> GSPGISGGGGGILSLLCVGVKKAKFDGAQEKFNTYVTLKVQNVESTTIAVRGSQPS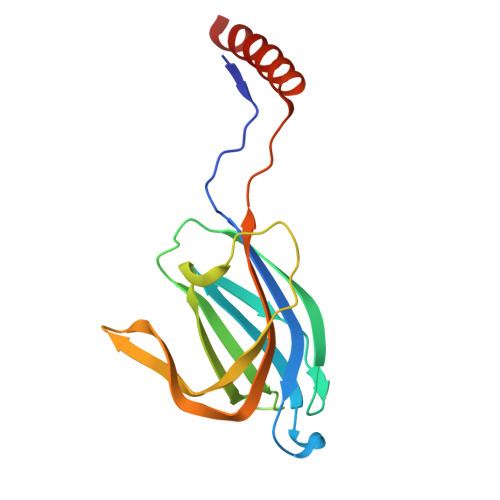WEQDFMFEINRLDLGLTVEVWNKGLIWDTMVGTVWIPLRTIRQSNEEGPGEWLTLDSQAIMADSEICGTKDPTFHRILLDAHFELPLDIPEEEARYWAKKLEQLNAKLNSS>[2x]DTKEQRILRYVQQNAKPGDPQSVLEAIDTYCTQKEWAMNVGDAKGQIMDAVIREYSPSLVLELGAYCGYSAVRMARLLQPGA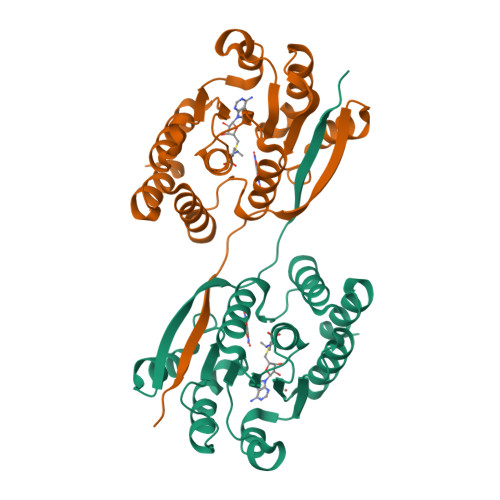RLLTMEMNPDYAAITQQMLNFAGLQDKVTILNGASQDLIPQLKKKYDVDTLDMVFLDHWKDRYLPDTLLLEKCGLLRKGTVLLADNVIVPGTPDFLAYVRGSSSFECTHYSSYLELMKVVDGLEKAIYQGP> GQESSTQRRADRKAQRDAERARLKAEQQAADAVSYDDAVAALKAQQFVLEANQVMFRNGQTAFVTSNTNFVLVNQGRGTVQVAFNTVYPGPNGIGGVTVDGTVSDIKTSTDKRG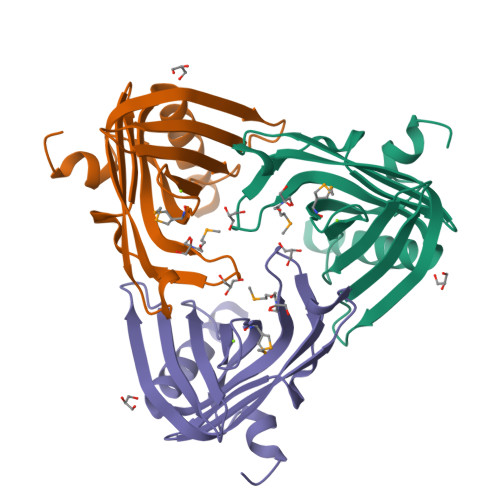NINCSFSIQGIGISAQIFLTLTNGDNNATVTINPNFNSNTMTLSGSLLPLNQSNIFKGRSW>[2x]EFPYYLRSFLVVLKTVLENEDDMLLFDEQEKGIVTKFYQLSATGQKLYVRLFQRKLSWIKMTKLEYEEIALDLTPVIEELTNAGFLQTESELQELSEVLELLSAPELKSLAKTFHLVNPNGQKQQLVDAFLKLAKQRSVCTWGK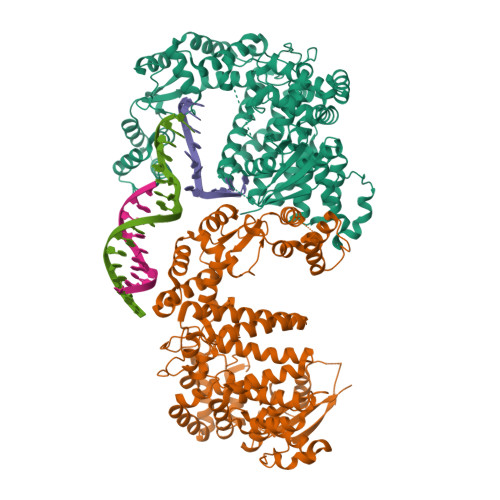NKPGIGAVILKRAKALAGQSVRICKGPRAVFSRILLLFSLTDSMEDEDAACGGQGQLSTVLLVNLGRMEFPSYTINRKTHIFQDRDDLIRYAAATHMLSDISSAMANGNWEEAKELAQCAKRDWNRLKNHPSLRCHEDLPLFLRCFTVGWIYTRILSRFVEILQRLHMYEEAVRELESLLSQRIYCPDSRGRWWDRLALNLHQHLKRLEPTIKCITEGLADPEVRTGHRLSLYQRAVRLRESPSCKKFKHLFQQLPEMAVQDVKHVTITGRLCPQRGMCKSVFVMEAGEAADPTTVLCSVEELALAHYRRSGFDQGIHGEGSTFSTLYGLLLWDIIFMDGIPDVFRNACQAFPLDLCTDSFFTSRRPALEARLQLIHDAPEESLRAWVAATWHEQEGRVASLVSWDRFTSLQQAQDLVSCLGGPVLSGVCRHLAADFRHCRGGLPALVVWNSQSRHFKLVEVKGPNDRLSHKQMIWLAELQKLGAEVEVCHVVAVGAKSQSLS> IAPTVWKLADRSKIYMADLESALHYILRIEVGRF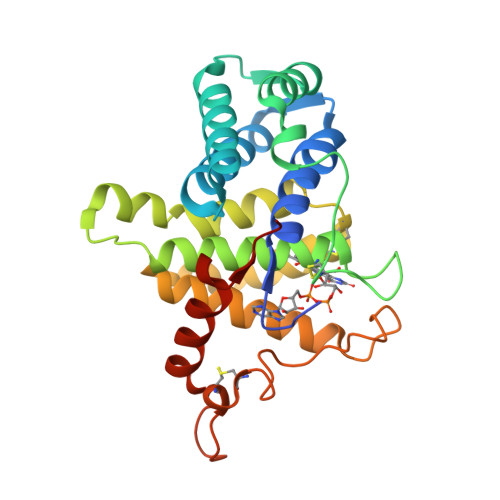PVLEGQRLVALKKFVAVLAKYFPGRPLVQNFLHSVNEWLKRQKRNKIPYSFFKTALDDRKEGAVLAKKVNWIGCQGSEPHFRGFPCSLWVLFHFLTVQAARQNVDHSQEAAKAKEVLPAIRGYVHYFFGCRDCASHFEQMAAASMHRVGSPNAAVLWLWSSHNRVNARLAGAPSEDPQFPKVQWPPRELCSACHNERLDVPVWDVEATLNFLKAHFSPSNIILDFPA> MDSAITLWQFLLQLLQKPQNKHMICWTSNDGQFKLLQAEEVARLWGIRKNKPNMNYDKLSRALRYYYVKNIIKKVNGQKFVYKFVSYPEILNM;>[2x]GA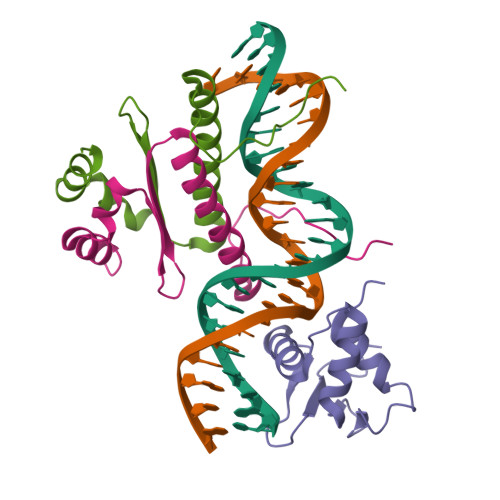KPGKKTRGRVKIKMEFIDNKLRRYTTFSKRKTGIMKKAYELSTLTGTQVLLLVASETGHVYTFATRKLQPMITSETGKALIQTCLNSPDSPPRSDPTTDQR> MGSSHHHHHHSQDPGFCFNILCVGETGLGKSTLMDTLFNTKFEGEPATHTQPGVQLQSNTYDLQESNVRLKLTIVSTVGFGDQINKEDS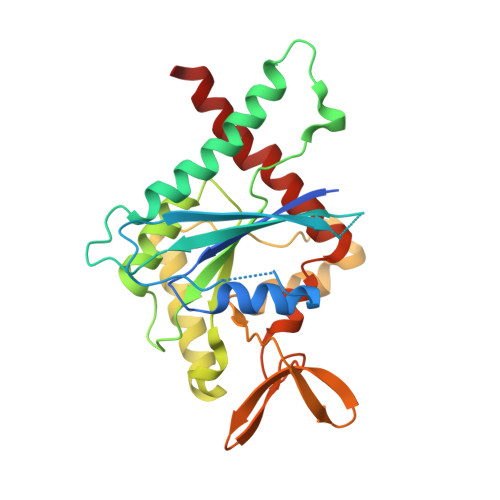YKPIVEFIDAQFEAYLQEELKIRRVLHTYHDSRIHVCLYFIAPTGHSLKSLDLVTMKKLDSKVNIIPIIAKADAISKSELTKFKIKITSELVSNGVQIYQFPTDDESVAEINGTMNAHLPFAVIGSTEELKIGNKMMRARQYPWGTVQVENEAHCDFVKLREMLIRVNMEDLREQTHTRHYELYRRCKLEE> GLPVYITPGSGQFMTTDDMQSPCALPWYHPTKEISIPGEVKNLIEMCQVDTLIPVN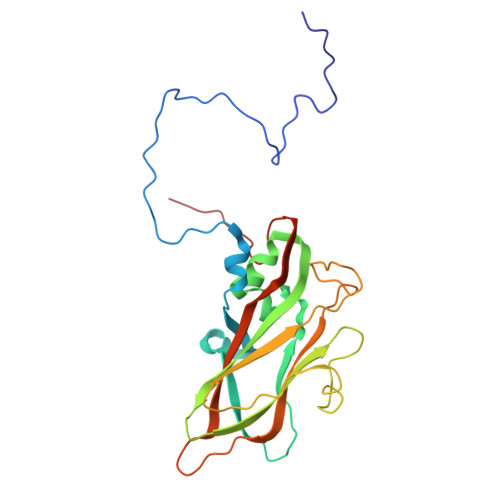NVGNNVGNVSMYTVQLGNQTGMAQKVFSIKVDITSTPLATTLIGEIASYYTHWTGSLRFSFMFCGTANTTLKLLLAYTPPGIDEPTTRKDAMLGTHVVWDVGLQSTISLVVPWVSASHFRLTADNKYSMAGYITCWYQTNLVVPPSTPQTADMLCFVSACKDFCLRMARDTDLHIQSGPIEQ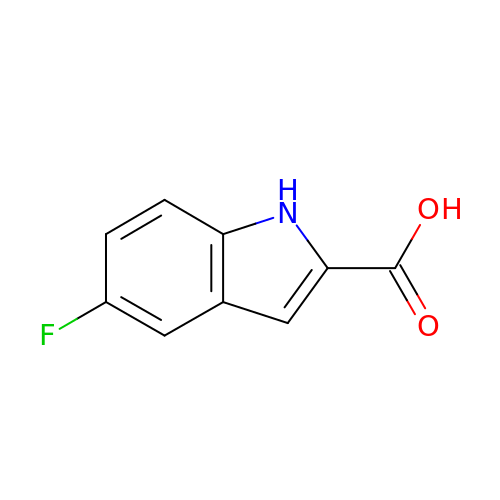5-fluoroindole-2-carboxylic acid | C9 H6 F N O2 | WTXBRZCVLDTWLP-UHFFFAOYSA-N>[2x]MVLERNETMYYGGSLWSPPSNWNPFTPWNAVPGTTGLVYETMFFYDPLTGNFDPWLAEKGEWLDSKTYRVVLREGIYWHDNVPLTSEDVRFTFEIAKKYKGIHYSSVWEWLDHIETPDNRTVIFVFKDPRYHEWNELLYTLPIVPKHIWEEKDE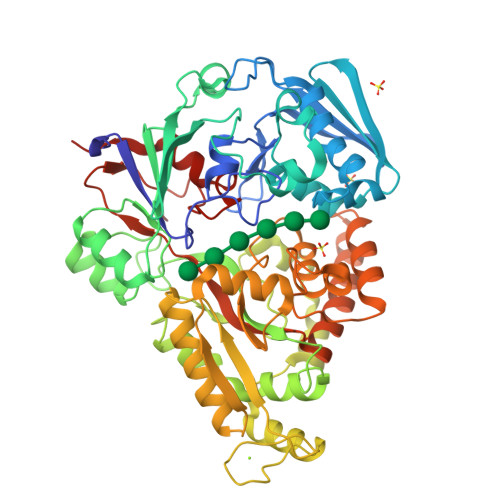TTILQSSNEYPLGSGPYVAHSWDQNKMIFERFENWWGTKVMGVKPAPKYVVIVRVLSNNVALGMLMKGELDFSNFMLPGVPILKKVYNLNTWYDEPPYHLSSTVVGLFLNARKYPLSLPEFRRAIAMSINADPIVQRVYEGAVLKADPLGFLPNSVWMKYYPKEVVEKHGFKYDPEEAKSILDKLGFRDVNGDGFRETPDGKPIKLTIECPYGWTDWMQAIQVIVDQLKVVGINAEPYFPDSSKYYENMYKGEFDIEMNANGTGISSTPWTYFNTIFYPDALESEFSYTGNYGRYQNPEVESLLEELNRTPLDNVEKVTELCGKLGEILLKDLPFIPLWYGAMAFITQDNVWTNWPNEHNPYAWPCGWANWWQTGALKILFNLKPAKHHHHHH>MEQAMRERSELARKGIARAKSVVALAYAGGVLFVAENPSRSLQKISELYDRVGFAAAGKFNEFDNLRRGGIQFADTRGYAYDRRDVTGRQLANVYAQTLGTIFTEQAKPYEVELCVAEVAHYGETKRPELYRITYDGSIADEPHFVVMGGTTEPIANALKESYAENASLTDALRIAVAALRAGSADTSGGDQPTLGVASLEVAVLDANRPRRAFRRITGSALQALLVDQESPQSDGESSG[14x];>[14x]TTIVALKYPGGVVMAGDRRSTQGNMISGRDVRKVYITDDYTATGIAGTAAVAVEFARLYAVELEHYEKLEGVPLTFAGKINRLAIMVRGNLAAAMQGLLALPLLAGYDIHASDPQSAGRIVSFDAAGGWNIEEEGYQAVGSGSLFAKSSMKKLYSQVTDGDSGLRVAVEALYDAADDDSATGGPDLVRGIFPTAVIIDADGAVDVPESRIAELARAIIESRSGADT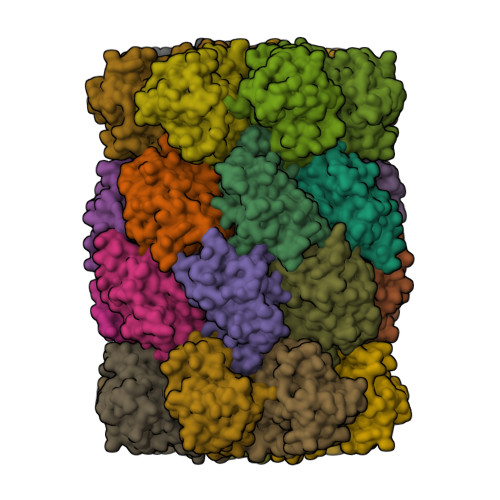FGSDGGEKHHHHHH>GGTATACC[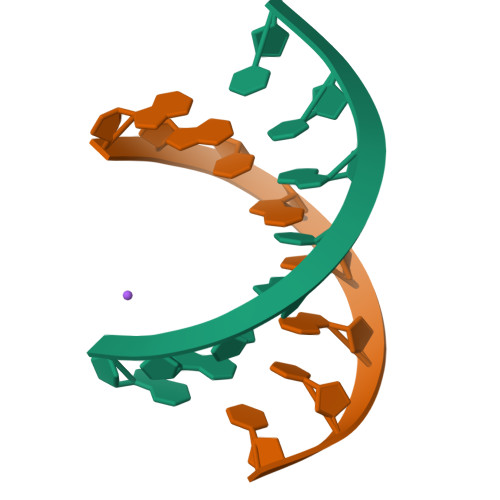2x]>[2x]RIPRIYHPISLENQTQCYLSEDAANHVARVLRMTEGEQLELFDGSNHIYPAKIIESNKKSVKVEILGRELADKESHLKIH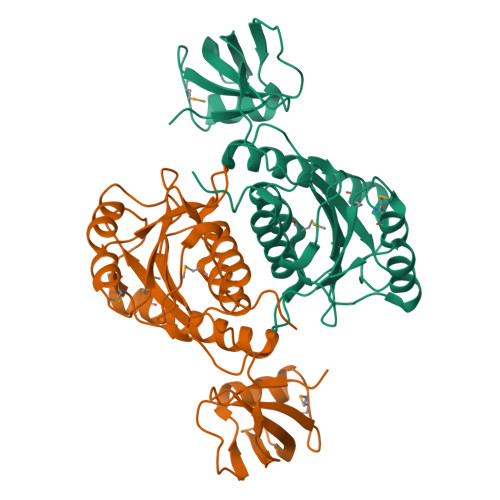LGQVISRGERMEFTIQKSVELGVNVITPLWSERCGVKLDAERMDKKIQQWQKIAIAACEQCGRNIVPEIRPLMKLQDWCAENDGALKLNLHPRAHYSIKTLPTIPAGGVRLLIGSEGGLSAQEIAQTEQQGFTEILLGKRVLRTETASLAAISALQICFGDLGEAA>MGRSHHHHHHGSLVPRGSEQGSNVNHLIKVTDQSITEGYDDSDGIIKAHDAEN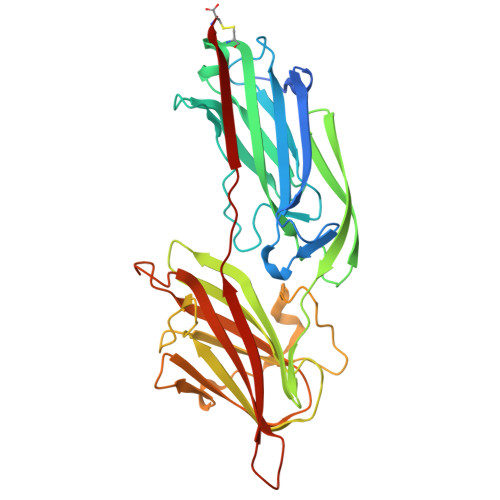LIYDVTFEVDDKVKSGDTMTVNIDKNTVPSDLTDSFAIPKIKDNSGEIIATGTYDNTNKQITYTFTDYVDKYCNIKAHLKLTSYIDKSKVPNNNTKLDVEYKTALSSVNKTITVEYQKPNENRTANLQSMFTNIDTKNHTVEQTIYINPLRYSAKETNVNISGNGDEGSTIIDDSTIIKVYKVGDNQNLPDSNRIYDYSEYEDVTNDDYAQLGNNNDVNINFGNIDSPYIIKVISKYDPNKDDYTTIQQTVTMQTTINEYTGEFRTASYDNTIAFSTSSGQGQGDLC[2x]> MELPRAFGLLLHPTSLPGPYGVGVLGREARDFLRFLKEAGGRYWQVLPLGPTGYGDSPYQSFSAFAGNPYLIDLRPLAERGYVRLEDPGFPQGRVDYGLLYAWKWPALKEAFRGFKEKASPEEREAFAAFREREAWWLEDYALFMALKGAHGGLPWNRWPLPLRKREEKALREAKSALAEEVAFHAFTQWLFFRQWGALKAEAEALGIRIIGDMPIFVAEDSAEVWAHPEWFHLDEEGRPTVVAGVPPDYFSETGQRWGNPLYRWDVLEREGFSFWIRRLEKALELFHLVRIAHFRGFEAYWEIPASCPTAVEGRWVKAPGEKLFQKIQEVFGEVPVLAEDLGVITPEVEALRDRFGLPGMKVLQFAFDNGMENPFLPHNYPAHGRVVVYTGTHNNDTTLGWYRTATPHEKAFMARYLADWGITFREEEEVPWALMHLGMKSVARLAVYPVQDVLALGSEARMNYPGRPS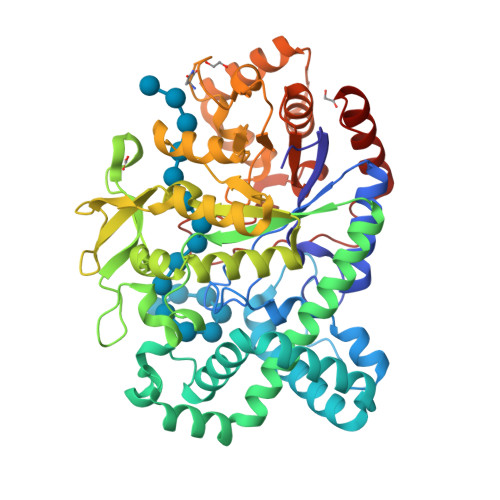GNWAWRLLPGELSPEHGARLRAMAEATERL> GHGHMHGRLKVKTSEEQAEAKRLEREQKLKLYQSATQAVFQKRQAGELDESVLELTSQILGANPDFATLWNCRREVLQHLETEKSPEESAALVKAELGFLESCLRVNP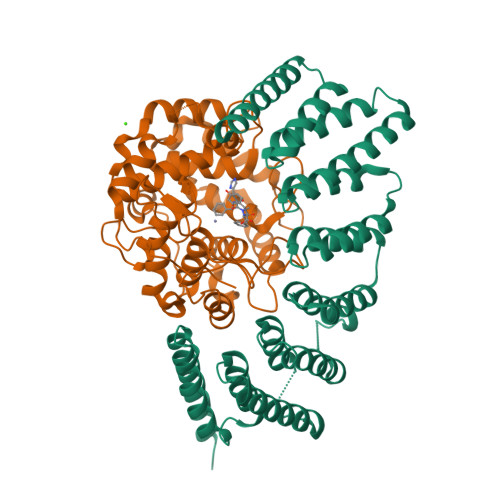KSYGTWHHRCWLLSRLPEPNWARELELCARFLEADERNFHCWDYRRFVAAQAAVAPAEELAFTDSLITRNFSNYSSWHYRSCLLPQLHPQPDSGPQGRLPENVLLKELELVQNAFFTDPNDQSAWFYHRWLLGAGSGRCELSVEKSTVLQSELESCKELQELEPENKWCLLTIILLMRALDPLLYEKETLQYFSTLKAVDPMRAAYLDDLRSKFLLENSVLKMEYA;> MGTQQKDVTIKSDAPDTLLLEKHADYIASYGSKKDDYEYCMSEYLRMSGVYWGLTVMDLMGQLHRMNKEEILVFIKSCQHECGGVSASIGHDPHLLYTLSAVQILTLYDSIHVINVDKVVAYVQSLQKEDGSFAGDIWGEIDTRFSFCAVATLALLGKLDAINVEKAIEFVLSCMNFDGGFGCRPGSESHAGQIYCCTGFLAITSQLHQVNSDLLGWWLCERQLPSGGLNGRPEKLPDVCYSWWVLASLKIIGRLHWIDREKLRSFILACQDEETGGFADRPGDMVDPFHTLFGIAGLSLLGEEQIKPVSPVFCMPEEVLQRVNVQPELVS One such multienzyme is propionyl-CoA carboxylase (PCC), which catalyzes the carboxylation of propionyl-CoA to form methylmalonyl-CoA, a precursor to the citric acid cycle intermediate succinyl-CoA. Propionyl-CoA carboxylase (PCC) is a multienzyme complex consisting of up to six α-subunits and six β-subunits. The α-subunit of LtPCC contains three domains: a biotin carboxylase (BC) domain, BC-CT mediating (BT) domain, and biotin carboxyl carrier protein (BCCP) domain. The β-subunit is composed of the structurally homologous N-carboxyltransferase (N-CT) and C-carboxyltransferase (C-CT) domains (Huang et al., 2010, Scheffen et al., 2021).

Here, we report three structures of endogenous LtPCC: an α6β6 dodecamer, α5β6 undecamer, and α4β6 decamer. To sort out LtPCCs with missing α-subunits, we performed symmetry-relaxed 3D classification and determined two additional LtPCC structures: α5β6 undecamer, α4β6 decamer. The α5β6 undecamer lacks one α-subunit, and the α4β6 decamer lacks two α-subunits on opposite sides of the LtPCC complex. In our decamer, undecamer, and dodecamer, the conformation of individual subunits is preserved. In other words, the structures of these complexes differ from one another only in the number and positioning of α-subunits. We utilize the α5β6 and α4β6 architectures of PCC to demonstrate that PCC oligomeric isomers differ only in the number of α-subunits. For each oligomeric isomer, the α-β binding site is either occupied or unoccupied. In other oligomeric isomers, at least one active site cannot participate in catalysis, and so all non-dodecameric PCCs are less catalytically active than the dodecamer. We found that most endogenous LtPCCs exist as α6β6, and in descending frequency, LtPCC also exhibit oligomeric isoforms with the oligomeric formulae α5β6, α4β6, α3β6, α2β6, α1β6, and α0β6.

>[5x]VLVANRGEIACRVMATCRRLGIKTVAVYSTADEQAKHVKVADESVCIGPPASVESYLCIDKIVDACKKTGAQAVHPGYGFLSENGEFQSALQKNNIVFVGPDAHSIESMGDKIESKRLAQRAGVTCIPGFIGEVKTHEDLLRFAREIGYPVMIKASGGGGGKGMRVAYNDTQCVEYYDMCREEAKAAFHSDKMLVERFIDHPRHIEIQVIADRRGNTVYLPERECSIQRRNQKVIEEAPSVLLDATTRKAMGEEAVAMARAVQYVSAGTVENVVNPQKQFYFLEMNTRLQVEHPITEEITGVDLVEQMLRAAADLPLSITQDDITINGHATECRVYAEDPMKNYFPSIGRLTMYQEPTGAGVRCDSGIIEGSQISVYYDPLICKLSTWGRDRAECIGRMEKALDEYVIRGLRHNICLLRDVVTEPRYRSGSITTNYLQEQYPNGFKKAELTAEEMQLMYEVAACVHLKRERLHYTQGTAPSERQLYLSVGAGQEGETPVYVRYLDDSHFEIGASKHGPFRKMEVVWKASYPIIRVKDGEAETVLQFWGTNEVTYGMQMRGTTFDVNVMSDLQSTLAHFVPITEATTNTKQILSPMPGVIVAIKVQPGQMVVAGEELLTLEAMKMRNKIHAQADGKVKEVKVKLGATVEDNEVLVELE;>[6x]PTAAEDLRHKKKRLTAMERVQLFCDPGTFRERDALVEHECHNFGMEKRKVPGDGFITGTGKVFGRPVFLFSHDFTVFGGSLSRTNAAKVVRIMEEAAKIGVPVIGFNDSGGARIHEGVDSLAGYADIFLRNTLFSGVIPQISVIMGPCAGGAVYSPAITDFTFMVETSSYMFVTGPEVVSAVGGKLVTKDELGGPHVHATKSGVSAGTFPNDIVAMAQLRRLYSYLPLSNRDPVPVLPTADERYRDVSSLNTVVPTEVKEAYDMRDVIYPVIDHDSFFEIQPQFAKNIICGFARVEGRSVCIIANQPKVQAGVLDIDSSVKGARMVRFADAFNIPIITFVDVPGFLPGVQQEYGGIIRHGAKLLYAYAEATVPKVTIITRKAYGGAYDVMSSKHLRGDSNYAWPHAEIAVMGAAGACKLLYSKETAEQQAQRIADYEKTFCTPLSAARKGFVDAVIDPSETRMRVCEDLERLARKQLQNPWKKHGNIPL> MTGVISSSSIGEKINEWYMYIRRFSIPDAEYLRREIKQELDQMEEDQDLHLYYSLMEFRHNLMLEYLEPLEKMRIEEQPRLSDLLLEIDKKQARLTGLLEYYFNFFRGMYELDQREYLSAIKFFKKAESKLIFVKDRIEKAEFFFKMSESYYYMKQTYFSMDYARQAYEIYKEHEAYNIRLLQCHSLFATNFLDLKQYEDAISHFQKAYSMAEAEKQPQLMGRTLYNIGLCKNSQSQYEDAIPYFKRAIAVFEESNILPSLPQAYFLITQIHYKLGKIDKAHEYHSKGMAYSQKAGDVIYLSEFEFLKSLYLSGPDEEAIQGFFDFLESKMLYADLEDFAIDVAKYYHERKNFQKASAYFLKVEQVRQLIQGGVSLYEIEV;> QRGMI

In Bacillus, the Rap protein family modulates complex signaling processes mediated by two-component systems, such as competence, sporulation, or biofilm formation, by inhibiting the RR components involved in these pathways. The second subgroup, comprising RapC, RapF, RapG, RapH, and RapK, blocks the action of the target RR by a direct interaction with their DNA binding domain, and works as an anti-activator. For Rap proteins, regulatory peptides are called Phr and their mature active form is a penta- or hexa-peptide generated from a ∼40 amino-acid precursor by means of a post-transcriptional export-import process. As previously disclosed by the crystal RapF structure in complex with the DNA-binding domain of its RR target ComA, RapF was an all-helical protein consisting of two domains: a small N-terminal 3-helix bundle domain (residues 1–68) and a large C-terminal TPR domain (residues 98–370), both connected by a linker region (69–97).

The RapF-PhrF structure reveals that the inhibitory peptide was bound to the TPR domain. PhrF lies in an extended conformation, as described for several TPR-peptide complexes, and interacted with the residues of six of the seven TPR repeats (TPR2–TPR7). In particular, the strictly conserved Asn in the RNPP superfamily, Asn227 in RapF, emerged from TPR4 to bind by a hydrogen bond with PhrF Met4, and a Rap family conserved TPR2 Tyr (Tyr152 in RapF) bound the main chain oxygen of PhrF Gly3. The C-terminal PhrF oxygens interacted with Arg223 (TPR4) by a salt bridge, and with Gln183 (TPR3) and Tyr66 (3-helix bundle) by both hydrogen bonds. On the opposite end, Asp338 from TPR7 was salt-bridged with N-terminal PhrF nitrogen. The side chain of PhrF Arg2 was situated in a hydrophobic pocket formed by Tyr152, Lys155 (both from TPR2), and Ala334 (TPR7), which was closed by the conserved Asp194 (TPR3), which interacted with Arg2 via a salt bridge. PhrF placed on the concave side of the RapF TPR channel, similarly to that observed for PlcR and PrgX, two RNPP representatives, in complex with their regulatory peptides (PapR and cCF10, respectively). Peptide binding to RapF induced a severe constriction in the TPR channel (volume lowered to 4,954 Å3) and a large displacement of the 3-helix bundle domain (see below), which partially closed one of the channel faces. The conformational changes proved even more drastic in the 3-helix bundle domain, which underwent a rotation of around 155° in relation to the position observed in the peptide-free RapF structures. The structures reported here confirm that the ComA and PhrF binding sites are independent and corroborate that PhrF mediates action allosterically by the conformational changes described in the previous section. All together, the partial disruption and sterical obstruction of the ComA binding site explain PhrF-induced RapF inhibition.>[2x]MTADELVFFVNGKKVVEKNADPETTLLVYLRRKLGLCGTKLGCGEGGCGACTVMISKYDRLQNKIVHFSVNACLAPICSLHHVAVTTVEGIGNTQKLHPVQERIARSHGSQCGFCTPGIVMSMYTLLRNQPEPTVEEIENAFQGNLCRCTGYRPILQGFRTFAKDGGCCGGSGNNPNCCMNQTKDQTVSLSPSLFNPEDFKPLDPTQEPIFPPELLRLKDTPQKKLRFEGERVTWIQASTMEELLDLKAQHPDAKLVVGNTEIGIEMKFKNMLFPLIVCPAWIPELNSVVHGPEGISFGASCPLSLVESVLAEEIAKLPEQKTEVFRGVMEQLRWFAGKQVKSVASIGGNIITASPISDLNPVFMASGAKLTLVSRGT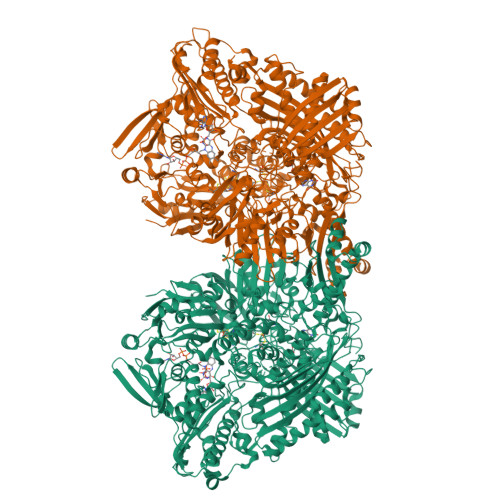RRTVRMDHTFFPGYRKTLLRPEEILLSIEIPYSKEGEFFSAFKQASRREDDIAKVTSGMRVLFKPGTIEVQELSLCFGGMADRTISALKTTPKQLSKSWNEELLQSVCAGLAEELQLAPDAPGGMVEFRRTLTLSFFFKFYLTVLQKLGRADLEDMCGKLDPTFASATLLFQKDPPANVQLFQEVPKDQSEEDMVGRPLPHLAANMQASGEAVYCDDIPRYENELSLRLVTSTRAHAKITSIDTSEAKKVPGFVCFLTAEDVPNSNATGLFNDETVFAKDEVTCVGHIIGAVVADTPEHAQRAARGVKITYEDLPAIITIQDAINNNSFYGSEIKIEKGDLKKGFSEADNVVSGELYIGGQEHFYLETNCTIAVPKGEAGEMELFVSTQNTMKTQSFVAKMLGVPDNRIVVRVKRMGGGFGGKETRSTVVSTALALAAHKTGRPVRCMLDRDEDMLITGGRHPFLAKYKVGFMKTGTVVALEVAHFSNGGNTEDLSRSIMERALFHMDNAYKIPNIRGTGRICKTNLPSNTAFRGFGGPQGMLIAEYWMSEVAITCGLPAEEVRRKNMYKEGDLTHFNQKLEGFTLPRCWDECIASSQYLARKREVEKFNRENCWKKRGLCIIPTKFGISFTLPFLNQGGALVHVYTDGSVLLTHGGTEMGQGLHTKMVQVASRALKIPTSKIHISETSTNTVPNTSPTAASASADLNGQGVYEACQTILKRLEPFKKKKPTGPWEAWVMDAYTSAVSLSATGFYKTPNLGYSFETNSGNPFHYFSYGVACSEVEIDCLTGDHKNLRTDIVMDVGSSLNPAIDIGQVEGAFVQGLGLFTMEELHYSPEGSLHTRGPSTYKIPAFGSIPIEFRVSLLRDCPNKRAIYASKAVGEPPLFLASSIFFAIKDAIRAARAQHGDNAKQLFQLDSPATPEKIRNACVDQFTTLCVTGVPENCKSWSVRI> DDKMDYDFKVKLSSERERVEDLFEYEGCKVGRGTYGHVYKAKRKDGKDDKDYALKQIEGTGISMSACREIALLRELKHPNVISLQKVFLSHADRKVWLLFDYAEHDLWHIIKFHRASKANKKPVQLPRGMVKSLLYQILDGIHYLHANWVLHRDLKPANILVMGEGPERGRVKIADMGFARLFNSPLKPLADLDPVVVTFWYRAPELLLGARHYTKAIDIWAIGCIFAELLTSEPIFHCRQEDIKTSNPYHHDQLDRIFNVMGFPADKDWEDIKKMPEHSTLMKDFRRNTYTNCSLIKYMEKHKVKPDSKAFHLLQKLLTMDPIKRITSEQAMQDPYFLEDPLPTSDVFAGCQIPYPKREFLTEEPPLKK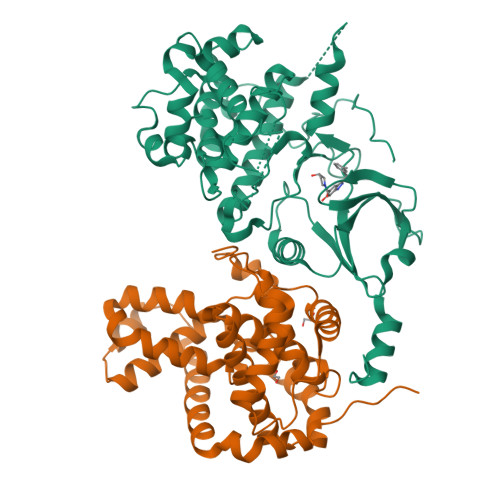;> KAMAGNFWQSSHYLQWILDKQDLLKERQKDLKFLSEEEYWKLQIFFTNVIQALGEHLKLRQQVIATATVYFKRFYARYSLKSIDPVLMAPTCVFLASKVEEFGVVSNTRLIAAATSVLKTRFSYAFPKEFPYRMNHILECEFYLLELMDCCLIVYHPYRPLLQYVQDMGQEDMLLPLAWRIVNDTYRTDLCLLYPPFMIALACLHVACVVQQKDARQWFAELSVDMEKILEIIRVILKLYEQWKNFDERKEMATILSKMPKPKPPP>[2x]MVKVAYVQMNPQILEPDKNYSKAEKLIKEASKQGAQLVVLPELFDTGYNFE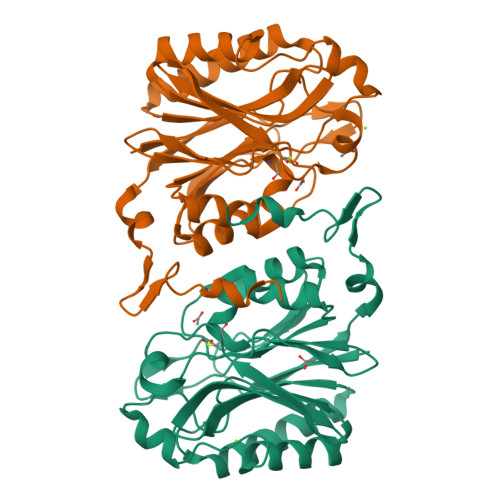TREEVFEIAQKIPEGETTTFLMDVARDTGVYIVAGTAEKDGDVLYNSAVVVGPRGFIGKYRKIHLFYREKFFFEPGDLGFRVFDLGFMKVGVMICFDWFFPESARTLALKGADVIAHPANLVMPYAPRAMPIRALENKVYTVTADRVGEERGLKFIGKSLIASPKAEVLSMASETEEEVGVAEIDLSLVRNKRINDLNDIFKDRREEYYFR> SQAFQRQLTALIGYDVTDVSNVHDDELEFTRRGLVTPRMAEVASRDPKLYAMHPWVTSKPLPEYLWKKIANNCIFIVIHRSTTSQTIKVSPDDTPGAILQSFFTKMAKKKSLMDIPESQSEQDFVLRVCGRDEYLVGETPIKNFQWVRHCLKNGEEIHVVLDTPPDPALDEVRKEEWPLVDDCTGVTGYHEQLTIHGKDHESVFTVSLWDCDRKFRVKIRGIDIPVLPRNTDLTVFVEANIQHGQQVLCQRRTSPKPFTEEVLWNVWLEFSIKIKDLPKGALLNLQIYCGKAPALSSKASAESPSSESKGKVQLLYYVNLLLIDHRFLLRRGEYVLHMWQISGKGEDQGSFNADKLTSATNPDKENSMSISILLDNYCHPIALPKHQPTPDPEGDRVRAEMPNQLRKQLEAIIATDPLNPLTAEDKELLWHFRYESLKHPKAYPKLFSSVKWGQQEIVAKTYQLLARREVWDQSALDVGLTMQLLDCNFSDENVRAIAVQKLESLEDDDVLHYLLQLVQAVKFEPYHDSALARFLLKRGLRNKRIGHFLFWFLRSEIAQSRHYQQRFAVILEAYLRGCGTAMLHDFTQQVQVIEMLQKVTLDIKSLSAEKYDVSSQVISQLKQKLENLQNSQLPESFRVPYDPGLKAGALAIEKCKVMASKKKPLWLEFKCADPTALSNETIGIIFKHGDDLRQDMLILQILRIMESIWETESLDLCLLPYGCISTGDKIGMIEIVKDATTIAKIQQSTVGNTGAFKDEVLNHWLKEKSPTEEKFQAAVERFVYSCAGYCVATFVLGIGDRHNDNIMITETGNLFHIDFGHILGNYKSFLGINKERVPFVLTPDFLFVMGTSGKKTSPHFQKFQDICVKAYLALRHHTNLLIILFSMMLMTGMPQLTSKEDIEYIRD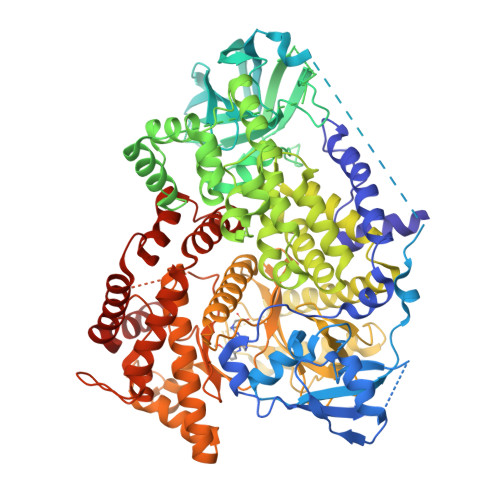ALTVGKNEEDAKKYFLDQIEVCRDKGWTVQFNWFLHLVLGIHHHHHH>MASRGSHHHHHHGAGDRGPEFPSSMPEESSPRRTPQSIPYQDLPHLVNADGQYLFCRYWKPTGTPK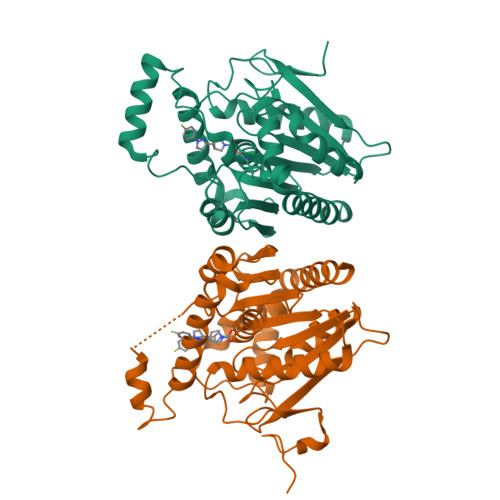ALIFVSHGAGEHSGRYEELARMLMGLDLLVFAHDHVGHGQSEGERMVVSDFHVFVRDVLQHVDSMQKDYPGLPVFLLGHSMGGAIAILTAAERPGHFAGMVLISPLVLANPESATTFKVLAAKVLNLVLPNLSLGPIDSSVLSRNKTEVDIYNSDPLICRAGLKVCFGIQLLNAVSRVERALPKLTVPFLLLQGSADRLCDSKGAYLLMELAKSQDKTLKIYEGAYHVLHKELPEVTNSVFHEINMWVSQRTATAGTASPPLEVDLQGDHGLSAWSHPQFEK[2x]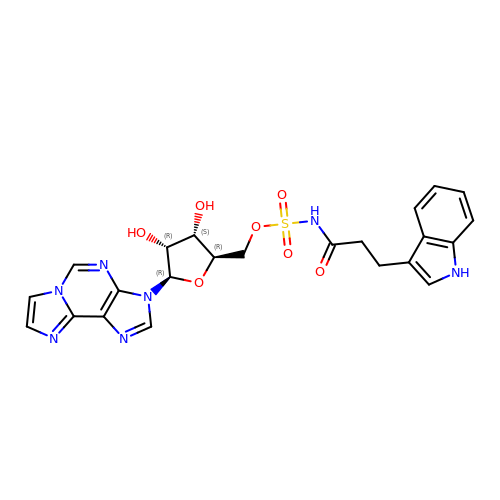3-(5-O-{[3-(1H-indol-3-yl)propanoyl]sulfamoyl}-beta-D-ribofuranosyl)-3H-imidazo[2,1-i]purine | C23 H23 N7 O7 S | QPCNFYXTDYZQFI-UGTJMOTHSA-N>[6x]MIPVTELRYFADTQPAYRILKPWWDVFTDYISIVMLMIAVFGGTLQVTQDKMICLPCKWVTKDSCNDSFRGWAASSPEPTYPNSTVLPTPDTGPTGIKYDLDRHQYNYVDAVCYENRLHWFAKYFPYLVLLHTLIFLACSNFWFKFPRTSSKLEHFVSILLKCFDSPWTTRALSETVVEESDPKPAFSKMNGSMDKKSSTVSEDVEATVPMLQRTKSRIEQGIVDRSETGVLDKKEGEQAKALFEKVKKFRTHVEEGDIVYRLYMRQTIIKVIKFALIICYTVYYVHNIKFDVDCTVDIESLTGYRTYRCAHPLATLFKI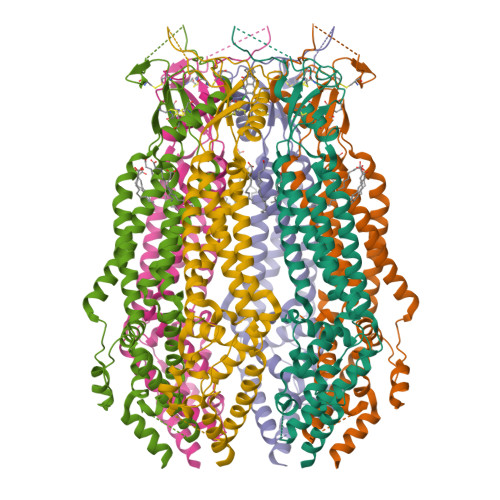LASFYISLVIFYGLICMYTLWWMLRRSLKKYSFESIREESSYSDIPDVKNDFAFMLHLIDQYDPLYSKRFAVFLSEVSENKLRQLNLNNEWTLDKLRQRLTKNAQDKLELHLFMLSGIPDTVFDLVELEVLKLELIPDVTIPPSIAQLTGLKELWLYHTAAKIEAPALAFLRENLRALHIKFTDIKEIPLWIYSLKTLEELHLTGNLSAENNRYIVIDGLRELKRLKVLRLKSNLSKLPQVVTDVGVHLQKLSINNEGTKLIVLNSLKKMVNLTELELIRCDLERIPHSIFSLHNLQEIDLKDNNLKTIEEIISFQHLHRLTCLKLWYNHIAYIPIQIGNLTNLERLYLNRNKIEKIPTQLFYCRKLRYLDLSHNNLTFLPADIGLLQNLQNLAVTANRIEALPPELFQCRKLRALHLGNNVLQSLPSRVGELTNLTQIELRGNRLECLPVELGECPLLKRSGLVVEEDLFSTLPPEVKERLWRADKEQASNSLEVLFQ> VESSTDGQVVPQE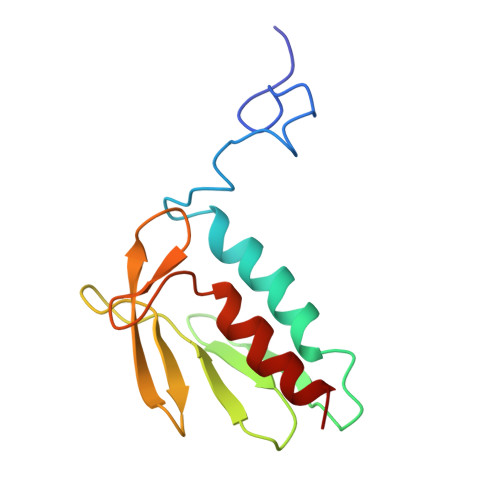VLNLPLEKAHEEADDYLDHLLDSLEELSEAHPDCIPDVELSHGVMTLEIPAFGTYVINKQPPNKQIWLASPLSGPNRFDLLNGEWVSLRNGTKLTDILTEEVEKAISK> MDVGQAVIFLGPPGAGKGTQASRLAQELGFKKLSTGDILRDHVARGTPLGERVRPIMERGDLVPDDLILELIREELAERVIFDGFPRTLAQAEALDRLLSETGTRLLGVVLVEVPEEELVRRILRRAELEGRSDDN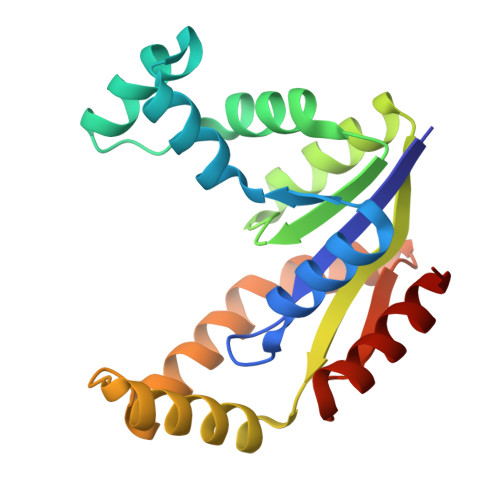EETVRRRLEVYREKTEPLVGYYEARGVLKRVDGLGTPDEVYARIRAALGI>[2x]MITVSIAGGSQPEILQLVKKALKEAEQPLQFIVFDTNENLDTENLWKYVHCSDEAAVAQEAVSLVATGQAQILLKGIIQTHTLLKEMLKSEHQLKNKPILSHVAMVELPAGKTFLLTDCAMNIAPTQATLIE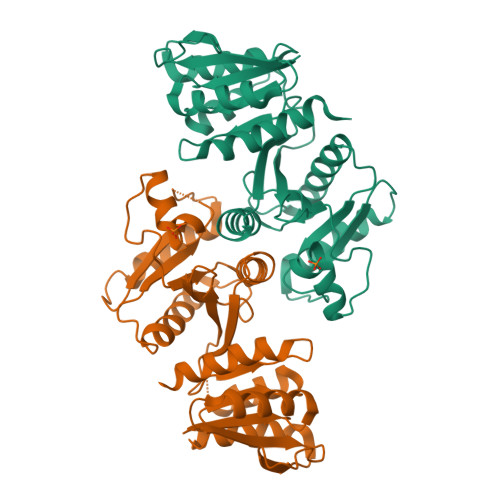IVENAKEVAQKLGLHHPKIALLSAAENFNPKMPSSVLAKEVTAHFNDQQEATVFGPLSLDLATSEEAVAHKRYSGPIMGDADILVVPTIDVGNCLYKSLTLFGHAKVGGTIVGTKVPVVLTSRSDSTESKFHSLRFAMRQVHHHHHH>MASVTEQFNDIISLYSTKLEHTSLRQDSPEYQGLLLSTIKKLLNLKTAIFDRLALFSTNETIDDVSTASIKFLAVDYYLGLLISRRQSNDSDVAQRQSMKLIYLKKSVESFINFLTLLQDYKLLDPLVGEKLGNFKDRYNPQLSELYAQPKNNKDLSGAQLKRKEK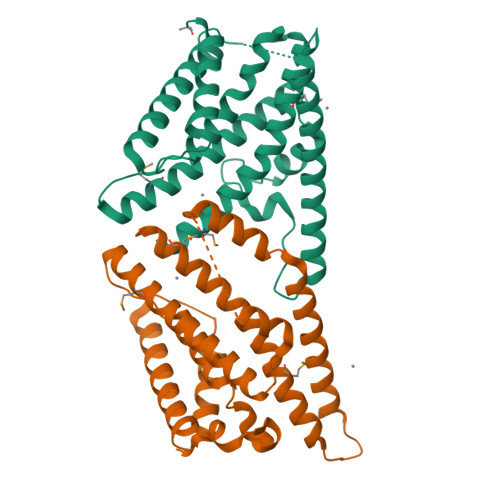IELFQRNKEISTKLHCLELELKNNDEDHDHDELLRELYLMRLHHFSLDTINNIEQNLFECEMLSNFLK[2x]3-benzyl-4-({[6-(cyclohexylmethyl)pyridin-2-yl]carbonyl}amino)benzoic 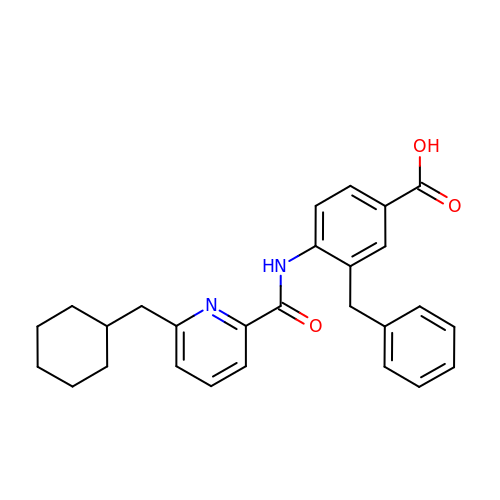acid | C27 H28 N2 O3 | QBZUPKMHCWADDF-UHFFFAOYSA-N>VLDGPYQPVTFKPPNDYWILINSNSNGVVLEGTNNTDVWVAIISIEPNVNSESRQYSLFGVNKQITVVNTSNKWKFMEMFRNNSNAEFQHKRTLTSSTKL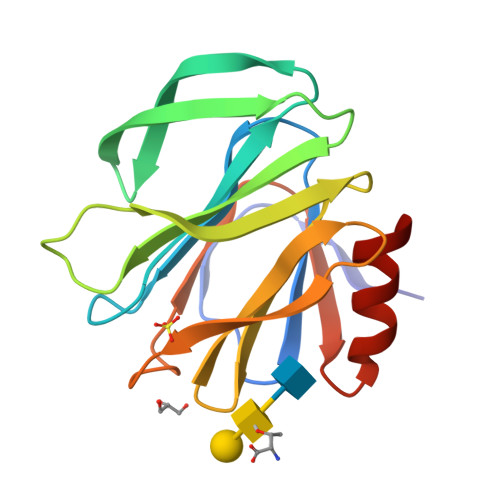VGILKHGGRLWTYHGETPNATTDYSTTSNLNEISVTTYAEFYIIPRSQESKCTEYINTGL[2x]>GLDTVSFSTKGATYITYVNFLNELRVKLKPEGNSHGIPLLRKKCDDPGKCFVLVALSNDNGQLAEIAIDVTSVYVVGYQVRNRSYFFKDAPDAAYEGLFKNTIKTRLHFGGSYPSLEGEKAYRETTDLGIE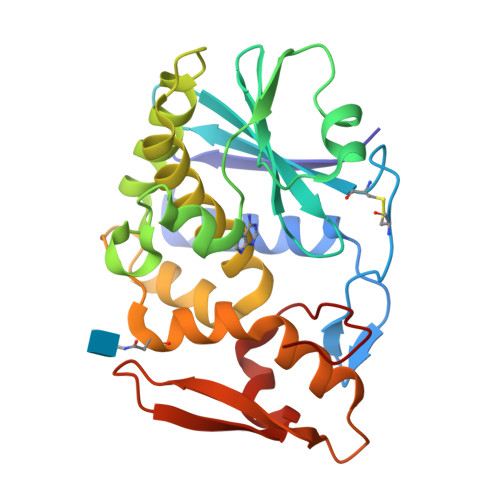PLRIGIKKLDENAIDNYKPTEIASSLLVVIQMVSEAARFTFIENQIRNNFQQRIRPANNTISLENKWGKLSFQIRTSGANGMFSEAVELERANGKKYYVTAVDQVKPKIALLKFVDKDPK[2x]>[3x]MKKRLTITL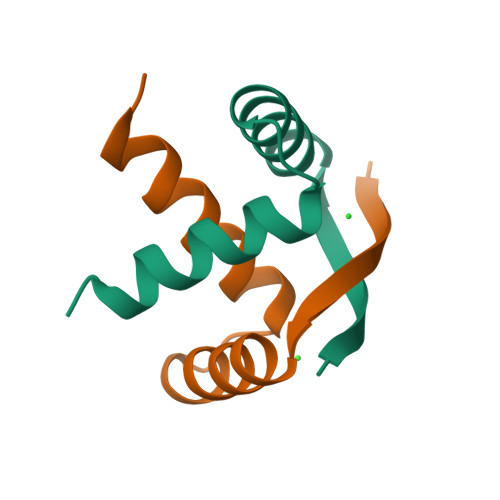SESVLENLEKMAREMGLSKSAMISVALENYKKGQER>MAESNALDKRLGELRLRADAGGPWARTFSERQQISNRHARAYDQTVSGLEIGLDRGWSASGGRWY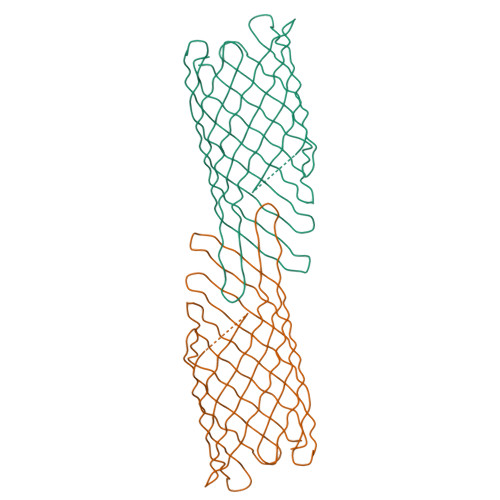AGGLLGYTYADRTYPGDGGGKVKGLHVGGYAAYVGDGGYYLDTVLRLGRYDQQYNIAGTDGGRVTADYRTSGAAWSLEGGRRFELPNDWFAEPQAEVMLWRTSGKRYRASNGLRVKVDANTATLGRLGLRFGRRIALAGGNIVQPYARLGWTQEFKSTGDVRTNGIGHAGAGRHGRVELGAGVDAALGKGHNLYASYEYAAGDRINIPWSFHAGYRYSF[3x]> AP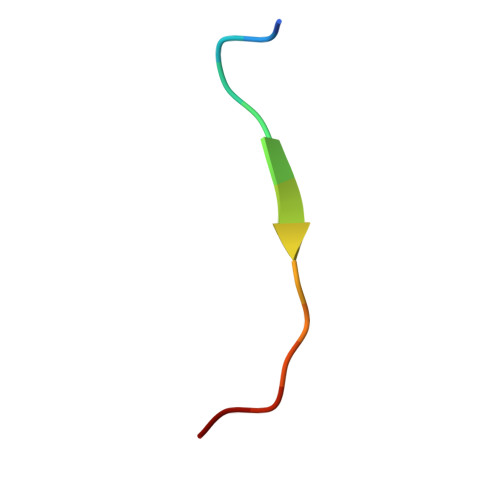STGGVIKPHRYR>MTTSINSVVTVFQNVFTNHGSTLLNGILIATTVGGQSLVRKLTFSCPCAYPLNIYHSLVFMFGPTAALLLIGITVNSTTWKLAHGFFFRVRDTRHSWKTTCVSWIEVLIQSSVAPIAWLFVVFLDGGYYRCYRSHEFCLISDAILCKNSTILNSYASTSSFNKISDNGKYCPPCICVPNPTDASYLEAESQIYAWGLLLFSGVAAFLVITCNRMCDKYTLVQRQYVETYKNVETQKFDAVAKEHASQLAEHNARAFFGQKDWTKRDWDWVSG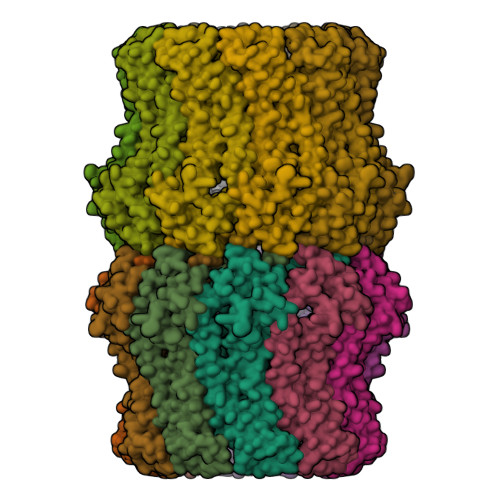IPEVNNPLFARLRLIAAEKTQQTMYTPLQLWNDNKGYRIPQPDLQLTQIIVDETKED[20x]>[4x]GPGSMAGKLEGRVAFITGAARGQGRAHAVRMAAEGADIIAVDIAGKLPSCVPYDPASPDDLSET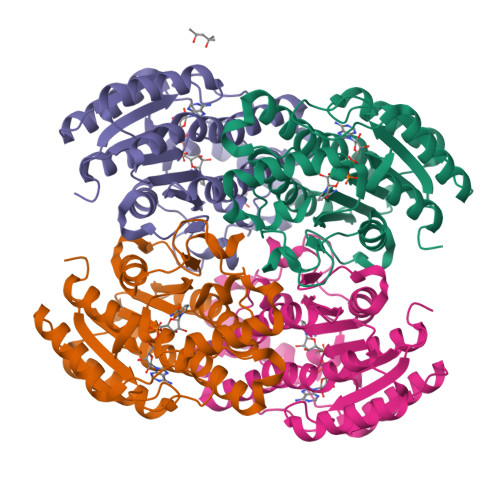VRLVEAANRRIVAAVVDTRDFDRLRKVVDDGVAALGRLDIIVANAGVAAPQAWDDITPEDFRDVMDINVTGTWNTVMAGAPRIIEGGRGGSIILISSAAGMKMQPFMIHYTASKHAVTGLARAFAAELGKHSIRVNSVHPGPVNTPMGSGDMVTAVGQAMETNPQLSHVLTPFLPDWVAEPEDIADTVCWLASDESRKVTAAQIPVDQGSTQY The Enterovirus (EV) genus of the Picornaviridae family contains notable viral pathogens that cause various animal and human diseases and are regarded as potential zoonotic threats. These small non-enveloped RNA viruses contain 60 copies each of the viral proteins VP1-4 arranged to form an icosahedral protein capsid. VP1-3 each comprise a β-barrel with extended surface loops and C-termini that form the outer capsid surface. The N-termini of VP1-3, as well as the whole of VP4 (N-terminal to VP2 in the VP0 precursor), form a network on the inner surface. Glutathione (GSH), an important cellular reducing agent, is a crucial co-factor for the morphogenesis of enteroviruses, including PV.

Since GSH was shown to effectively stabilise wt PV2 VLPs they were soaked with a molar excess of the benzene sulphonamide derivative CP17 (VLP:CP17 molar ratio of 1:2500), applied to grids and vitrified for single-particle cryo-EM. After image processing, a final set of 51,518 particles yielded a 1.97 Å icosahedral reconstruction for the wt PV2-CP17 complex (FSC 0.143). Like the binding mode for GSH, CP17 is bound within the VP1–VP3 interprotomer pocket of the wt PV2 VLP through two critical arginine residues—Arg243 and Arg258—from neighbouring VP1 subunits, which form hydrogen bonds and salt-bridges with the carboxylate group of CP17. The bulk of CP17 forms hydrophobic interactions with the network of residues forming the VP1–VP3 interprotomer pocket of the wt PV2 VLP. The wt PV2-CP17 structure is similar to that of the CVB3-CP17 complex (RMSD in Cα atoms of 1.1 Å), but there are differences in the precise orientation of CP17 as bound to wt PV2 VLP and CVB3 virus, although the key charge interactions with the carboxylate group of CP17 are maintained in both cases. In the wt PV2-CP17 complex, the compound lies flat due to sequence differences between PV2 and CVB3, where VP1-Phe76 in CVB3 is replaced by VP1-Ile89 in wt PV2. The interaction of the C-terminal residue VP3-Phe236 in CVB3 is absent in the wt PV2-CP17 structure as the C-terminus of VP3 is disordered in the latter, the final observed residue in wt PV2 being VP3 Ala235. In total 520 Å2 of solvent-accessible surface area for CP17 is buried in the interprotomer surface pocket of the wt PV2 VLP, representing ~87% of the total solvent-accessible surface area of the molecule. Interestingly, the greater bulk of CP17 means that the C-terminal residues of VP3, which becomes ordered on GSH binding remains disordered upon binding of CP17.

> GLGDLIEGVVEGVTRNALTPLTPANNLPDTQSSGPAHSKETPALTAVETGATNPLVPSDTVQTRHVIQKRTRSESTVESFFARGACVAIIEVDNDAPTKRASKLFSVWKITYKDTVQLRRKLEFFTYSRFDMEFTFVVTSNYTDANNGHALNQVYQIMYIPPGAPIPGKWNDYTWQTSSNPSVFYTYGAPPARISVPYVGIANAYSHFYDGFAKVPLAGQASTEGDSLYGAASLNDFGSLAVRVVNDHNPTKLTSKIRVYMKPKHVRVWCPRPPRAVPYYGPGVDYKDGLAPLPEKGLTTY;> MGAQVSSQKVGAHENSNRAYGGSTINYTTINYYRDSASNAASKQDFAQDPSKFTEPIKDVLIKTAPTLNSPNIEACGYSDRVMQLTLGNSTITTQEAANSVVAYGRWPEYIKDSEANPVDQPTEPDVAACRFYTLDTVTWRKESRGWWWKLPDALKDMGLFGQNMFYHYLGRAGYTVHVQCNASKFHQGALGVFAVPEMCLAGDSTTHMFTKYENANPGEKGGEFKGSFTLDTNATNPARNFCPVDYLFGSGVLAGNAFVYPHQIINLRTNNCATLVLPYVNSLSIDSMTKHNNWGIAILPLAPLDFATESSTEIPITLTIAPMCCEFNGLRNITVPRTQ;> GLPVLNTPGSNQYLTADNYQSPCAIPEFDVTPPIDIPGEVRNMMELAEIDTMIPLNLTNQRKNTMDMYRVELNDAAHSDTPILCLSLSPASDPRLAHTMLGEILNYYTHWAGSLKFTFLFCGSMMATGKLLVSYAPPGAEAPKSRKEAMLGTHVIWDIGLQSSCTMVVPWISNTTYRQTINDSFTEGGYISMFYQTRVVVPLSTPRKMDILGFVSACNDFSVRLLRDTTHISQEAMPQ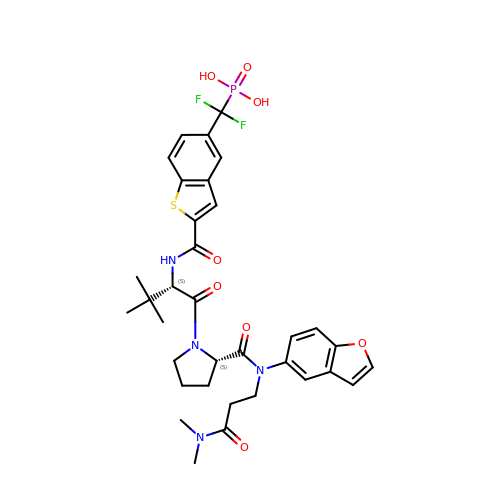N-{5-[difluoro(phosphono)methyl]-1-benzothiophene-2-carbonyl}-3-methyl-L-valyl-L-prolyl-N~3~-(1-benzofuran-5-yl)-N,N-dimethyl-beta-alaninamide | C34 H39 F2 N4 O8 P S | UTADYHXHDMKUES-PWUYWRBVSA-N> MDEKSTKIIMWLKKMFGDKPLPPYEVNTRTMEILYQLAEWNEARDKDLSLVTEDLKLKSAEVKAEAKYLQDLLTEGLGPSYTNLSRMGNNYLNQIVDSCLALELKNSSLSSYIPAVNDLSSELVAIELNNQEMEAELTSLRKKLTEALVLEKSLERDLKKAEEQCNFEKAKVEIRSQNMKKLKDKSEEYKYKIHAAKDQLSSAGMEEPLTHRSLVSLSETLTELKAQSMAAKEKLNSYLDLAPNPSLVKVKIEEAKRELKATEVELTTKVNMMEFVVPEPSKRRLK;> MSGGDRFVQTLQKLNYPKGAQLDGEDFDWLFEAVDLKPFLDWFCSAASEQ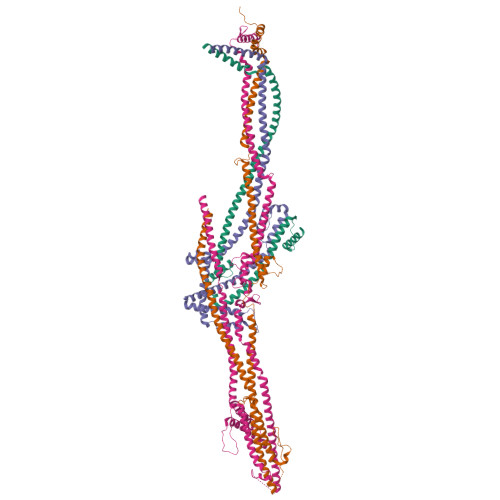NVVPDEKLQAFNTLKESGKPVLDEKALDEVLKTFSISKVPAIEEVAIEKLEEEVKALQKQKNLHIRRRNKLQMVESGNRQMCLKSKDKEEETGRAFQEVLHLLRVTNKKLNHELQSIVNGVQTLMSFFSTPETACELSSQPIFLSQLLLDKYLSLEEQSTAALTSFTKEHFFEGMSKFVEGSDENFQLVQLNVNSFGEDGTTEDKCKEMMRLQLAYICAKHKLIQMKAKSASLKVGLQWAENNASVVQDKASQKEENLKVRITSLKNETLQIENHTNSISNEKLPGLVRDNAQLLNMPIVKGDYDLQMAHQTSCSSRQDLVCDHLMKQKASFELLQLGYELELRKHRDVYRELGSIVQELKESGDKLEERLTMLSDVNLLSASKPRSNIDSKDLTSHRLYQLLDGDNTQKLFRTYDGLESVAQKLSQDIASMRDQLEVSEQEHSLLLSKLDSHLKELRDFMYPEGNTLMLTTPELSGEFHQLGSQLEKLNHITVEILGDLQLKRKMLESNKLQQIEKQLYVYFFQNEEQLKSIVGKLEAQTGGGSSA;> MAQTLQYVSSRLSMLQIDEEDLERNAQFGKVLIELCPLLGPNGGSANLNRELEETRRELLLQRKMWMRSEVIYQLVQEMLLDLQVRKLEGSLTEEERKFQDGLQQCMLVSECSRLLTADSVPPSDSTSILGLDKQDLLDLLPPNMLVLWVRDRLQKQLEEALKKKCFTFLSFHQPETDEEGDVLRAAKVLRLASTLEDEKRRLQNEQEKHQEMRALLEKQQEIYPHVLLRCLSLLRQAASELRLRAQSDIDRINAEYLEAKSNALFLKLRMEELQVLTDCYTPEKVLVHRQIRDTLEAGVKKEKQELSTSRQILSSYEFLGPEFEGLVQEYTRLKDKIKDNRWMLQELSKSLP;> MERRSLAQELKKWAVEEMGLPAQKAPSEEMLQRLFIGQCGDIWKFIIRHIHSHRTVRKIEGNLLWYQQLQHTEAQRTAEEEQQQRRKQLCKEILELRAELHHLQEQIQTAEREIVGQDLNCERAQDLCRRSLLLRAFNKKREEECEALCQSNKKIQYRCEQLQEIRRASQREVMFSAVDPDLSSSTFLEPEVLRDVREVCKLRFKFLRSLHDDSISSSVHPGKEDLRSLSHQQWMSMAEKVWNTHTPNHILAALERLTLNSTQELKKLQFSQAADLSKGPSCQLKEFSEPITQSRSCNESTHLDPQETLPSFHSLIQEGWANSVKVSSELRRVQSQAQALSEHLAERIQEIHKKLSDGSEVSVLTRAAFDAELRCVILRGCRDALMQECRMLQEEAAGKKQEMKLLQQQQQNIQEACLLLDKKQKHIQILIKGNSSSKSQIRRSSVEAQKYVQDKLLPWPQEIIQESQRLQDSIQKEVKHFSAICLPALLKVSTDGFNLLPSRELSINRMSNTHAPYYGIFKGIYESVRLPLYKAPESVLSHVADMKKQLFFLRSQLSSRSEAISKTQRALQKNTNPDTDALLKSLSDHYSLELDEMVPKMQRLIQQCEKHQEYGKEVQATVMDWWEQPVQLCLPSEERGGLTLRQWRERWTVAVTALQRATGSRS> VVGGEDAKPGQFPWQVVLNGKVDAFCGGSIVNEKWIVTAAHCVETGVKITVVAGEHNIEETEHTEQKRNVIRIIPHHNYNAAINKYNHDIALLELDEPLVLNSYVTPICIADKEYTNIFLKFGSGYVSGWGRVFHKGRSALVLQYLRVPLVDRATCLRSTKFTIYNNMFCAGFHEGGRDSCQGDSGGPHVTEVEGTSFLTGIISWGEECAMKGKYGIYTKVSRYVNWIKEKTKLT;> MDVTCNIKNGRCEQFCKNSADNKVVCSCTEGYRLAENQKSCEPAVPFPCGR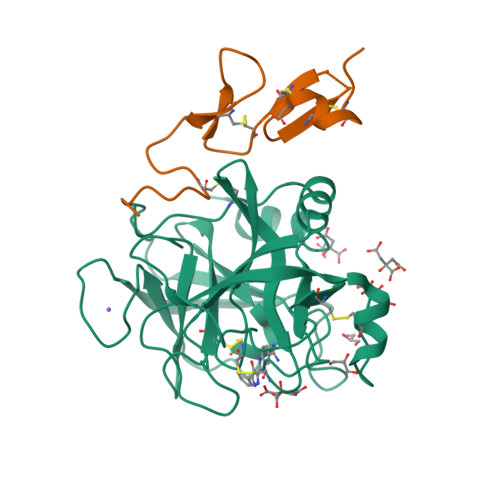VSVSQTSKLTR>[4x]FDYDGPLMKTEVPGPRSRELMKQLNIIQNAEAVHFFCNYEESRGNYLVDVDGNRMLDLYSQISSIPIGYSHPALVKLVQQPQNVSTFINRPALGILPPENFVEKLRESLLSV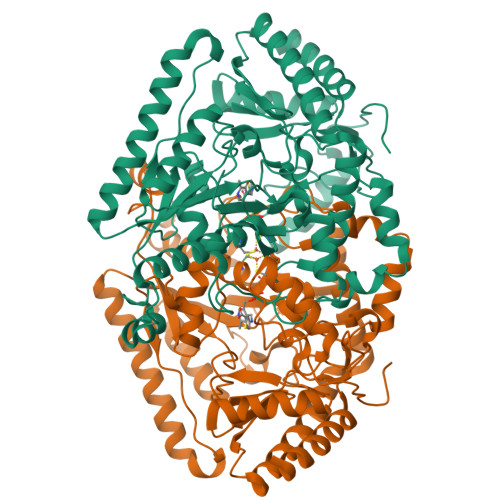APKGMSQLITMACGSCSNENAFKTIFMWYRSKERGESAFSKEELETCMINQAPGCPDYSILSFMGAFHGRTMGCLATTHSKAIHKIDIPSFDWPIAPFPRLKYPLEEFVKENQQEEARCLEEVEDLIVKYRKKKKTVAGIIVEPIQSEGGDNHASDDFFRKLRDISRKHGCAFLVDEVQTGGGSTGKFWAHEHWGLDDPADVMTFSKKMMTGGFFHKEEFRPNAPYRIFNTWLGDPSKNLLLAEVINIIKREDLLSNAAHAGKVLLTGLLDLQARYPQFISRVRGRGTFCSFDTPDESIRNKLISIARNKGVMLGGCGDKSIRFRPTLVFRDHHAHLFLNIFSDILADF> MAQFAFESDLHSLLQLDAPIPNAPPARWQRKAKEAAGPAPSPMRAANRSHSAGRTPGRTPGKSSSKVQTTPSKPGGDRYIPHRSAAQMEVASFLLSKENQPENSQTPTKKEHQKAWALNLNGFDVEEAKILRLSGKPQNAPEGYQNRLKVLYSQKATPGSSRKTCRYIPSLPDRILDAPEIRNDYYLNLVDWSSGNVLAVALDNSVYLWSASSGDILQLLQMEQPGEYISSVAWIKEGNYLAVGTSSAEVQLWDVQQQKRLRNMTSHSARVGSLSWNSYILSSGSRSGHIHHHDVRVAEHHVATLSGHSQEVCGLRWAPDGRHLASGGNDNLVNVWPSAPGEGGWVPLQTFTQHQGAVKAVAWCPWQSNVLATGGGTSDRHIRIWNVCSGACLSAVDAHSQVCSILWSPHYKELISGHGFAQNQLVIWKYPTMAKVAELKGHTSRVLSLTMSPDGATVASAAADETLRLWRCFELDPARRREREKASAAKSSLIHQGIR;> RAPXGDISN

Here we explore peptide inhibitors of Cdc20, a substrate-recognition subunit and activator of the E3 ubiquitin ligase the anaphase-promoting complex/cyclosome (APC/C) that is essential in mitosis and consequently of interest as an anti-cancer target. APC/C engages substrates via degrons that include the ‘destruction box’ (D-box) motif. The D-box binding site comprises a cleft between two of the beta-propeller blades and the neighbouring APC/C subunit APC10, which is thought to result in stabilisation of the active complex. We used a rational design approach to construct binders containing unnatural amino acids aimed at better filling a hydrophobic pocket that contributes to the D-box binding site on the surface of Cdc20.

We incorporated (S)–2-amino-4,4-dimethylpentanoic acid (C3) into the backbone sequences of D4, D10, and D19 replacing leucine at position 4, yielding peptides D7, D12, and D20, respectively. As expected, the structure–activity relationship (SAR) held true between all peptides, whereby incorporation of the unnatural amino acid increased the binding affinity over 6-fold versus the respective parental peptide. We attempted these soaking experiments with our four highest affinity peptides, D21, D20, D7, and D19 (in order of highest affinity to lowest) and were able to observe sufficient ligand density for all but D19. The crystal structures of Cdc20WD40 in complex with each of the other three D-box peptides show that they bound to Cdc20WD40 at the canonical D-box degron binding site, with a largely similar topology to the S. cerevisiae Acm1-Cdh1 structure (overlay of D21 with Acm1 D-box). The nitrogen backbone atom of the (S)–2-amino-4,4,4-trifluorobutanoic acid/(S)–2-amino-4,4-dimethylpentanoic acid unnatural amino acids also forms a hydrogen bond with the carbonyl of Asp177. All peptides form a hydrogen bond between the carbonyl of A2 to the amine of G5/S5. Interestingly, the observed electron density of the peptide correlates with Cdc20 binding affinity: D21 and D20, having the highest affinities, display the clearest electron density allowing six amino acids to be modelled, whereas D7 shows relatively poor density permitting modelling of only four residues. We then explored whether the D-box peptides at a fixed concentration stabilise the Cdc20, and for D7, D20, and D21 we observed increases in the thermal stability of Cdc20 that correlated with their binding affinities as previously determined.> MTIRHHVSDALLTAYAAGTLSEAFSLVVATHLSLCDECRARAGALDAVGGSLMEETAPVALSEGSLASVMAQLDRQIQRPAPARRADPRAPAPLADYVGRRLEDVRWRTLGGGVRQAILPTGGEAIARLLWIPGGQAVPDHGHRGLELTL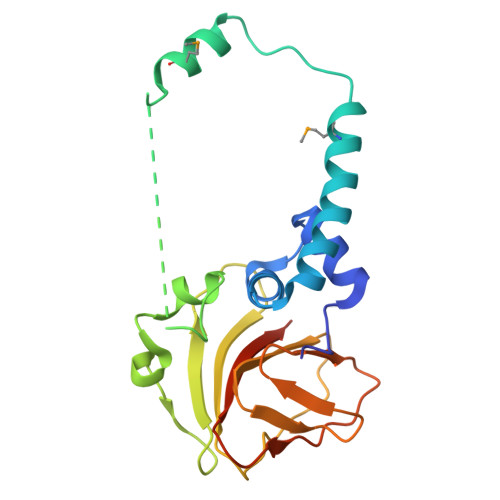VLQGAFRDETDRFGAGDIEIADQELEHTPVAERGLDCICLAATDAPLRFNSFL>[6x]SNASNS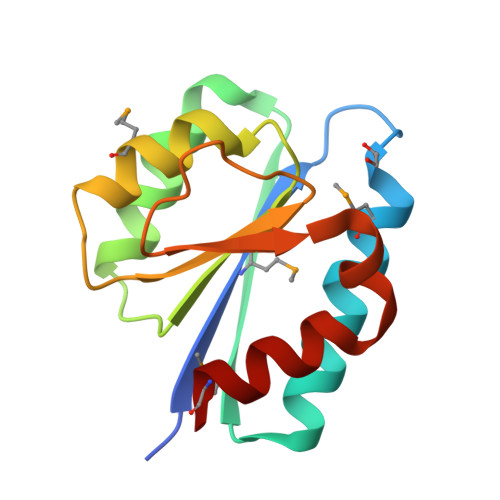KKSVSMILDIEGTNNEAMNNSALLALNNAQKKLNIDTNKVESDDSSTFSNSIDILCNDNYDLIIAVGARFAKPLEMVAKKYPKQQFAIIDYEYDKQPSNITSISYEDNKSGYLAGLIAGKMT> ELYTPKHEAGVCTFYEECGKNPELSGGLTSLSNVSCLSNTPARHVTGEHLALLQRICPRLYNGPNTTFACCSTKQLLSLESSMSITKALLTRCPACSDNFVSLHCHNTCSPDQSLFINVTRVVERGAGEPPAVVAYEAFYQRSFAEKAYESCSQVRIPAAASLAVGSMCGVYGSALCNAQRWLNFQGDTGNGLAPLDITFHLLEPGQALPDGIQPLNGKIAPCNESQGDDSAVCSCQDCAASCPVIPPPEALRPSFYMGRMPGWLALIIIFTAVFVLLSAVLVRLRVVSNRNKNKAEGPQEAPKLPHKHKLSPHTILGRFFQNWGTRVASWPLTVLALSFIVVIALAAGLTFIELTTDPVELWSAPKSQARKEKSFHDEHFGPFFRTNQIFVTARNRSSYKYDSLLLGSKNFSGILSLDFLLELLELQERLRHLQVWSPEAERN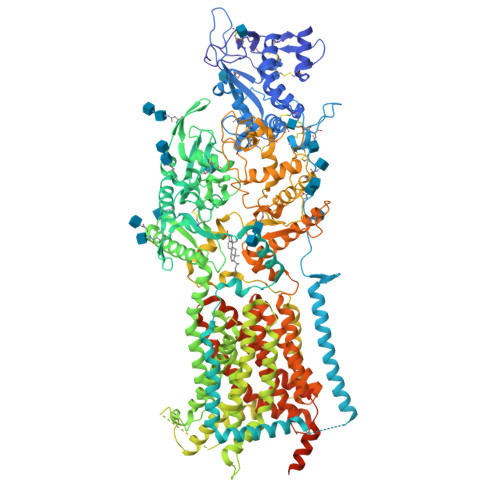ISLQDICYAPLNPYNTSLSDCCVNSLLQYFQNNRTLLMLTANQTLNGQTSLVDWKDHFLYCANAPLTFKDGTSLALSCMADYGAPVFPFLAVGGYQGTDYSEAEALIITFSLNNYPADDPRMAQAKLWEEAFLKEMESFQRNTSDKFQVAFSAERSLEDEINRTTIQDLPVFAVSYIIVFLYISLALGSYSRCSRVAVESKATLGLGGVIVVLGAVLAAMGFYSYLGVPSSLVIIQVVPFLVLAVGADNIFIFVLEYQRLPRMPGEQREAHIGRTLGSVAPSMLLCSLSEAICFFLGALTPMPAVRTFALTSGLAIILDFLLQMTAFVALLSLDSKRQEASRPDVLCCFSTRKLPPPKEKEGLLLRFFRKIYAPFLLHRFIRPVVMLLFLTLFGANLYLMCNINVGLDQELALPKDSYLIDYFLFLNRYLEVGPPVYFVTTSGFNFSSEAGMNATCSSAGCKSFSLTQKIQYASEFPDQSYVAIAASSWVDDFIDWLTPSSSCCRLYIRGPHKDEFCPSTDTSFNCLKNCMNRTLGPVRPTAEQFHKYLPWFLNDPPNIRCPKGGLAAYRTSVNLSSDGQVIASQFMAYHKPLRNSQDFTEALRASRLLAANITADLRKVPGTDPNFEVFPYTISNVFYQQYLTVLPEGIFTLALCFVPTFVVCYLLLGLDMCSGILNLLSIIMILVDTIGLMAVWGISYNAVSLINLVTAVGMSVEFVSHITRSFAVSTKPTRLERAKDATVFMGSAVFAGVAMTNFPGILILGFAQAQLIQIFFFRLNLLITLLGLLHGLVFLPVVLSYLGPDVNQALVQEEKLASEAAVAPEPSCPQYPSPADADANVNYGFAPELAHGANAARSSLPKSDQKFENLYFQGDYKDDDDKHHHHHHHHHH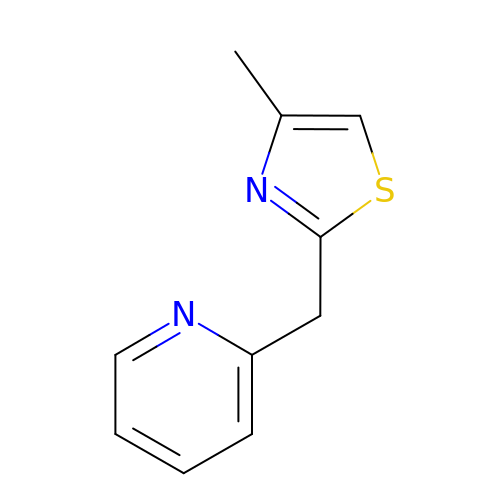2-[(4-methyl-1,3-thiazol-2-yl)methyl]pyridine | C10 H10 N2 S | YKMZZWADKYKWAT-UHFFFAOYSA-N> S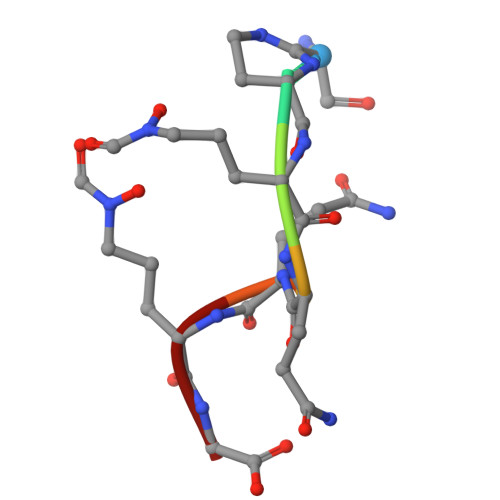AKQQKG> MWADEEPAPWDIEETPAEQAPEASAESAAPAAEAATGEKPKIKLEKIEPPHYNHHWVRPLFLNYAYYLYEYRKNYYNDVIDYLNQREKGIFREPPRAQEWAERAMRTYDEKNTDKSFKRSADMKYIINMRHEPRYYSYHTRAYYSLKYQKIL

Here, we report a thick filament structure from the indirect flight muscles of a third insect order, Hymenoptera, the Asian bumble bee Bombus ignitus. Flightin is essential for maintaining insect flight muscle structure and performance; when flightin is eliminated in Drosophila flight muscle myofibrils, defective myofilaments are formed and flight is severely impaired. Flightin sequences vary in length but have a strictly conserved region in the middle, dubbed the WYR motif that spans over ~50 amino acids that are critical for normal flightin function. The C-terminus is embedded within the backbone based on evidence that deletion of the C-terminus results in filaments of irregular length, whereas deletion of the N-terminus produces filaments of normal length but in flies that cannot fly.

The non-myosin protein flightin reveals a newly resolved extension at the C-terminus that overlaps a previously unassigned density in both Drosophila and Lethocerus. Here with Bombus, we observe for the first time what appears to be the complete density of the part of flightin embedded within the thick filament from the C-terminus deep within the backbone to residue 41, the first part of flightin stabilized by contact with the proximal S2. The shape of this density strongly supports its assignment to flightin due to the presence of a folded domain in the middle in the predicted position of the “WYR” motif. For flightin, AlphaFold2 predicted a reasonable atomic model for the WYR domain corresponding to residues 56 to 102. The model of the two ends of the flightin density was rebuilt de novo using Coot. The density corresponding to the residues on the N-terminal side of the WYR motif of Bombus flightin, similar to that of Lethocerus and Drosophila, passes between the myosin tails of one curved layer to reach the outside of the backbone. The WYR motif itself is situated at the inside of the myosin tail annulus, where it contacts two curved myosin layers. The density on the C-terminal side of the WYR motif passes across a pair of myosin tails of one curved layer and ends up contacting yet another curved layer on the N-terminal side. Flightin’s interaction with five different curved layers possibly explains its impact on determining filament length. Our more complete density of flightin resolves the identity of the so-called “blue” density first seen in Lethocerus thick filaments and later in Drosophila.>[2x]MEKRMSTQQRAAGNACPTAAFSFDPARLAQRRRWAGAFAALCGLALSPSALLAEEHSQHQDHAVELAPSVVTGVAQSSPLTIVTNPKEPRQPVPASDGADYLKTIPGFAVIRNGGSNGDPVLRGMFGSRLNILTNGGMMLGACPNRMDAPTSYISPETYDKLTVIKGPQTVLWGPGASAGTILFEREPERFGELGSRVNASLLAGSNGRFDKVLDAAAGNRLGYLRFTGNHAQSDDYEDGAGNTVPSRWKKWNGDVAVGWTPDEDTLIELTAGKGDGEARYAGRGMDGSQFKRESLGLRFVKSNVSDVLEKVEAQVYYNYADHIHDNFRLRTPDPSSMMPMPMASQVDRRTLGGRLAATWRWDDFKLVTGVDAMRNEHRARGSKYDMMTDYYTDADQFPWSKDAVFHNYGAFGELTWFAAERDRLIGGLRLDRASVKDYRQTLKSGHMGHAMANPTANDTRADTLPSGFVRYEHDLADSPTTLYAGLGHAERFPDYWELFSPKRGPNGSVNAFDKIKPEKTTQLDFGLQYNGDKLQAWASGYVGVVQDFILFSYREGMMGSSTQATNVDARIMGGELGASYQLTGNWKTDASLAYAWGKNSSDDRALPQIPPLEARFGLTYEEGDWSAGSLWRVVAPQNRIARDQGNVVGKDFDKSAGFGVFSLNGAYRVTRNVKLSAGVDNLFDKDYTEHLNKAGDAGFGFSANETVPEPGRTFWTKVDFSF

Here, we show that Pseudomonas aeruginosa OprC is an outer membrane, TonB-dependent transporter that is conserved in many Proteobacteria and which mediates acquisition of both reduced and oxidised ionic copper via an unprecedented CxxxM-HxM metal binding site. As indicated by the successful structure solution, OprC contains a single bound copper and shows the typical fold of a TBDT, with a large 22-stranded β-barrel occluded by an N-terminal approximately 15 kDa plug domain that, like in other TBDTs, completely occludes the lumen of the barrel. The copper binding site comprises residues Cys143 and Met147 in the plug domain and His323 and Met325 in the barrel wall. The CxxxM-HxM configuration, which coordinates the copper in a tetrahedral manner, is highly unusual and has, to our knowledge, not been observed before in copper homeostasis proteins.

Interestingly, the active site His117 in azurin renders the copper atom solvent inaccessible, reminiscent to the likely role of Met147 in OprC. The superficial similarity of the OprC binding site to that of (pseudo)azurin prompted us to generate the M147H and M325H OprC mutants in an attempt to convert OprC into a unique, blue copper transport protein. However, in the presence of added Cu(II), both mutants remain colourless, and comparison of the crystal structures with those of pseudoazurin and plastocyanin show small but most likely important differences in the geometries of the active sites.> AEGEIKVELEDSDDVAAACELRAQLAGVSIASG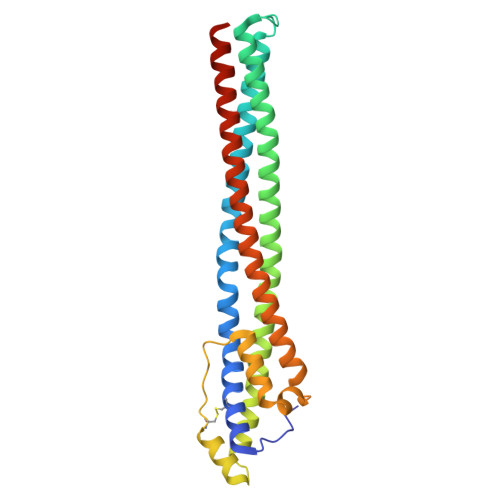ILLRPAVIRNATTEFSRKKSEDILAKGGAAVERASAAVDRVSGLDKTNETAQKVRKAAAVAHHALEHVKEEVEIVAKKVNEIIELTAGATEHAKGAKANGDASAVKVSNLLARAKESENQYVKEAAEECSESTNYDVTAKSLAAALDKLPGVKEDNAVKTTFQSILTSLDNLDKDVKSVEQRAEELETALEKAERQLEKAEKAAEEAETESSKVETESS>GPLGSELSRQIKAAASTLEDIEVKDDEWAVDMSEEAIRARAKELEVNSELTQLDEYGEWILEQAGEDKENLPSDVELYKKAAELDVLNDPKIGCVLAQCLFDEDIVNEIAEHNAFFTKILVTPEYEKNFMGGIERFLGLEHKDLIPLLPKILVQLYNNDIISEEEIMRFGTKSSKKFVPKEVSKKVRRAAKPFITWLETAESDDDEEDDE[2x];> GPLGSGSGDDLFAGLKKKKKKSKSVSADAEAEKEPTDDIAEALGELSLKKKKKKTKDSSVD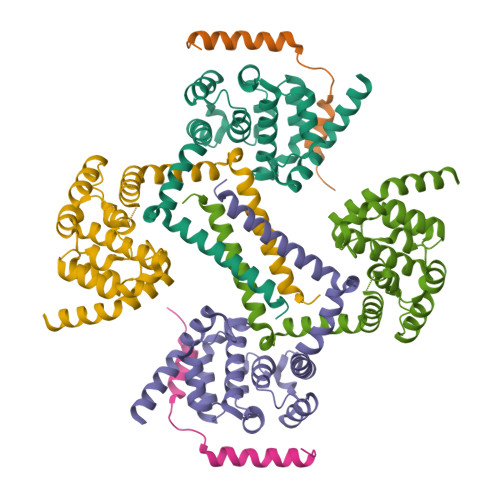AFEKELAKAGLD>[2x]AMDLELSMSETLTLPVLPLEDGVVLPGMVVPLDLSENGEVRAAIEAARAAAQSRGPGIRSVSKPRVLLVPRLNGRYADVGTLGVIE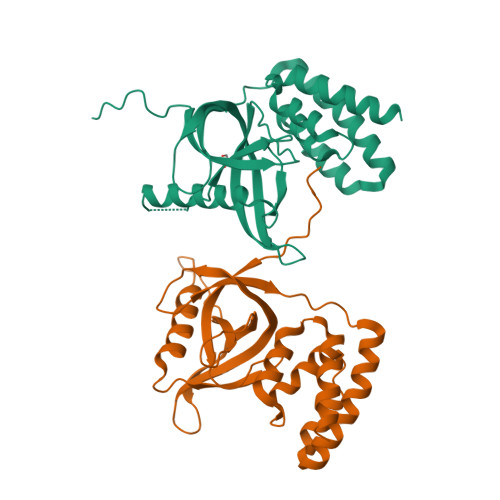QEGRLPGGEPGAVVRGVSRVRIGTGTTGPGAALWVEGTVLEAPPASGRAQELAKEYKGLVSAILQKRGAWQVVDVVQQIDDPSTLADNSGYAPYLTDEQKIEVLETVDVVERLELVIGWTRDHLAE Chuangxinmycin (CXM) is a promising antimicrobial compound targeting bacterial tryptophanyl-tRNA synthetase (TrpRS), an essential enzyme in protein synthesis. TrpRS catalyzes the ligation of Trp to its cognate tRNA, forming tryptophanyl-tRNA (Trp-tRNA), which is required for the accurate translation of genetic codes into proteins. Importantly, bacterial TrpRS exhibits significant structural and functional differences compared to its mammalian counterpart, making it an attractive target for the development of selective antibiotics. Structurally, CXM is a tryptophan (Trp) mimic but is characterized by a unique dihydrothiopyran heterocycle, which distinguishes it from other known antibiotics and contributes to its distinct physicochemical properties.

To investigate the tolerance of the TrpRS pocket, two analogues of CXM, 3-demethylchuangxinmycin (dCXM) and 3-methylchuangxinmycin (mCXM), were tested. The complex structures of these analogues with EcTrpRS and SaTrpRS were solved. All analogue complexes are isomorphous with the corresponding CXM complexes (ESI†), and the binding modes are nearly identical (ESI†). The flexibility of dCXM leads to diverse conformations across the three chains of the SaTrpRS/dCXM complex. Consistent with its more flexible conformation and reduced hydrophobic surface area, dCXM demonstrates significantly lower inhibitory activity compared to CXM.

>METLFSGIQPSGIPTIGNYIGALKQFVDVQNDYDCYFCIVDQHAITMPQDRLKLRKQTRQLAAIYLASGIDPDKATLFIQSEVPAHVQAGWMLTTIASVGELERMTQYKDKAQKAVEGIPAGLLTYPPLMAADIVLYNTNIVPVGDDQKQHIELTRNLVDRFNSRYNDVLVKPEIRMPKVGGRVMSLQDPTRKMSKSDDNAKNFISLLDEPNVAAKKIKSAVTDSDGIIKFDRDNKPGITNLISIYAGLTDMPIKDIEAKYEGEGYGKFKGDLAEIVKAFLVEFQEKYESFYNSDKLDDILDQGRDKAHKVSFKTVKKMEKAMGLGRKRHHHHHH[3x]>GIDPFTFENATSDAINQDMMLYIERIAKIIQKLPKRVHINVRGFTDDTPLVKTRFKSHYELAANRAYRVMKVLIQYGVNPNQLSFSSYGSTNPIAPNDSLENRMKNNRVEIFFSTDANDLSKIHSILDNEFNPHKQQE[12x]

The motility protein B (MotB) is a key component of the bacterial flagellar motor. It anchors the MotA/MotB stator ring of the motor to peptidoglycan (PG) of the cell wall and forms part of the proton-conducting channel that couples proton flow to generation of the turning force via an as yet unknown mechanism. The PG-binding site of MotB resides on the periplasmic C-terminal domain (MotB-C) which shows sequence similarity to outer membrane protein A (OmpA) and related PG-binding proteins. Although the PG-binding grooves formed by these loops are topologically very similar in different OmpA-like proteins, all five conserved residues (Gly161, Asp164, Leu179, Arg183, Arg226) that are thought to be essential for PG recognition are buried and inaccessible.

The structure of previously unobserved crystal form (Form B) of recombinant H. pylori MotB-C was solved by a molecular replacement approach using AMORE. The asymmetric unit of the form B crystal contains 12 subunits. The overall fold of each monomer is very similar to the Form A structure. It contains a mixed four-stranded β-sheet, with three α-helices packing against one face of it, and the fourth forming an N-terminal extension of one of the β-strands. The three longer petal-like loops (β1α1 (residues 126–133), β2α2 (163–174) and β3β4 (207–225)) have been previously implicated in the PG binding by MotB and PG-associated lipoprotein (PAL). Structural analysis and calculations of the accessible side-chain surface area in Form A and Form B crystals of H. pylori MotB-C and in the crystal structure of the periplasmic domain of Salmonella MotB show that all five conserved residues are clustered on one side of the molecule and are completely shielded from the solvent by loops (β1α1), (β2α2) and (β3β4). The most significant differences are observed in the structures of loops β1α1, β2α2 and β3β4 at the PG binding site, with the following residues showing the largest displacements of Cα atoms: Glu126 (2.3 Å), Asn127 (2.4 Å) (loop β1α1), Val169 (2.8 Å), Lys170 (4.1 Å) (loop β2α2) and Asp216 (2.4 Å) (loop β3β4). Analysis of the distribution of the main-chain temperature factor averaged over the total of 12 monomers in the asymmetric units of the Form B crystals also highlights these three loops as the most variable regions in the structure. Structure superimposition shows that there are significant differences in conformations of many side chains and the orientation of the main-chain peptide groups in loops β1α1, β2α2 and β3β4. Thus, our crystallographic analysis suggests that the flexibility of the semi-conserved loop region β1α1, β2α2 and β3β4 is important for PG-binding activity of MotB.> GSKHDGRVKIGHYVLGDTLGVGTFGKVKIGEHQLTGHKVAVKILNRQKIRSLDVVGKIKREIQN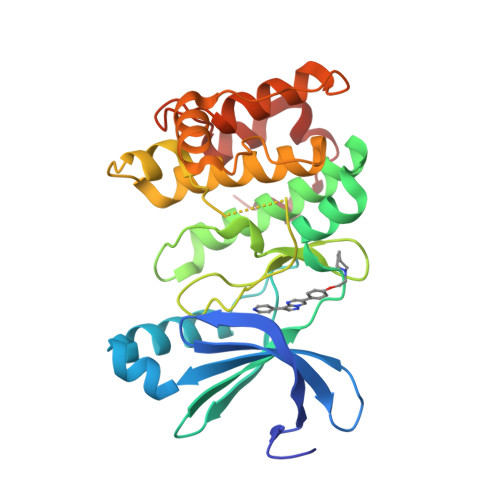LKLFRHPHIIKLYQVISTPTDFFMVMEYVSGGELFDYICKHGRVEEMEARRLFQQILSAVDYCHRHMVVHRDLKPENVLLDAHMNAKIADFGLSNMMSDGEFLRDSCGSPNYAAPEVISGRLYAGPEVDIWSCGVILYALLCGTLPFDDEHVPTLFKKIRGGVFYIPEYLNRSVATLLMHMLQVDPLKRATIKDIREHEWFKQDLPSYLFPE Since only far-red light is available at a deep layer of the colony, P. crispa has evolved a molecular system for photosystem II (PSII) excitation using far-red light with uphill energy transfer. Here, we purified a light-harvesting chlorophyll (Chl)-binding protein complex from P. crispa (Pc-frLHC) that excites PSII with far-red light and revealed its ring-shaped structure with undecameric 11-fold symmetry at 3.13 Å resolution. The primary structure suggests that Pc-frLHC evolved from LHCI rather than LHCII. The circular arrangement of the Pc-frLHC subunits is unique among eukaryote LHCs and forms unprecedented Chl pentamers at every subunit‒subunit interface near the excitation energy exit sites.

Pc-frLHC is an undecamer with 11-fold symmetry. Pc-frLHC is the first example of a ring-shaped eukaryotic LHC. On the other hand, subunit‒subunit interactions in Pc-frLHC are strengthened by the long N-terminal regions of the subunit. The long N-terminal region of every Pc-frLHC subunit interacts with the N-terminal regions of both sides of the subunits in the ring-shaped structure. We found 11 Chls and two carotenoids in the subunit of Pc-frLHC. We, therefore, modeled the 11 Chls as Chl a. The vio and loro in the all-trans configuration were assigned in the L1- and L2-binding sites of Pc-frLHC, respectively. Chl708 and 603 are located side by side, and Chl609 makes stacking (π‒π) interactions with Chl708 and 603; Chl603, 609, and 708 form a unique trimeric structure. Instead, Pc-frLHC has His171, and this His residue coordinates directly the Mg2+ of Chl708. Moreover, the ring-shaped arrangement of 11 subunits in Pc-frLHC enables Chl708 to interact with the Chl613’-614’ dimer in the adjacent subunit, forming a Chl pentamer that may contribute to further red shift absorption.

>[11x]MAPYSVVASVLAAAPPQQSGSVRQLPSTINRAITQRSQSRHVASASSASSPTTMLEERDNLWEIGGPYWWPFSSFTPPAHLDGSLPGDRGFDPFSLGTSWGQPPVDVSDPNYDESRLRWLLEGELYNGRLAMLAVVGVLTVEAQGKGPWWEIPGNLNLFGTPYVVAVVGGHLAFALLEKKRLENFRETGEAGHFGAARFDPLDLTEANPLGTDYNRQAEVRNCRLAMLTFLGFSVQAWVTGKGPIENAKDHLASPFEANIFTYGDRGTNVVAIFSAFAAVMHIAELAREKKAEDKPRSRNRTLSGSS> LGSNTH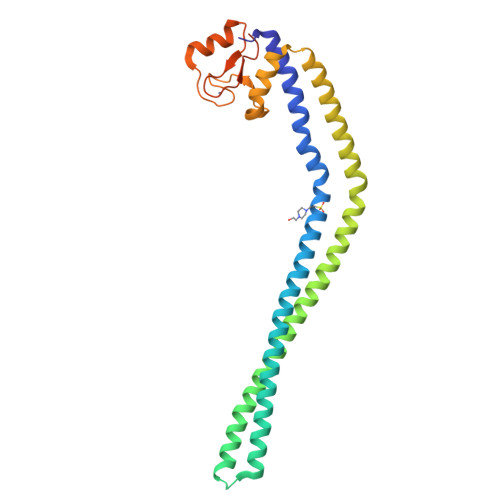LKQLIEISHLDKEIDSLEPLIREKRKDLDKALNDKEAKNKAILNLEEEKLALKLQVSKNEQTLQDTNAKIASIQKKMSEIKSERELRSLNIEEDIAKERSNQANREIENLQNEIKRKSEKQEDLKKEMLELEKLALELESLVENEVKNIKETQQIIFKKKEDLVEKTEPKIYSFYERIRRWAKNTSIVTIKKQACGGCFIRLNDKIYTEVLTSGDMITCPYCGRILYAEGAYESNAQPPKESQEESQELV>[2x]MHELTIYHFMSDKLNLYSDIGNIIALRQRAKKRNIKVNVVEINETEGITFDECDIFFIGGGSDREQALATKELSKIKTPLKEAIEDGMPGLTICGGYQFLGKKYITPDGTELEGLGILDFYTESKTNRLTGDIVIESDTFGTIVGFENHGGRTYHDFGTLGHVTFGYGNNDEDKKEGIHYKNLLGTYLHGPILPKNYEITDYLLEKACERKGIPFEPKEIDNEAEIQAKQVLIDRANRQKKSRLEHHHHHH;>MRQWTAIHLAKLARKASRAVGKRGTDLPGQIAR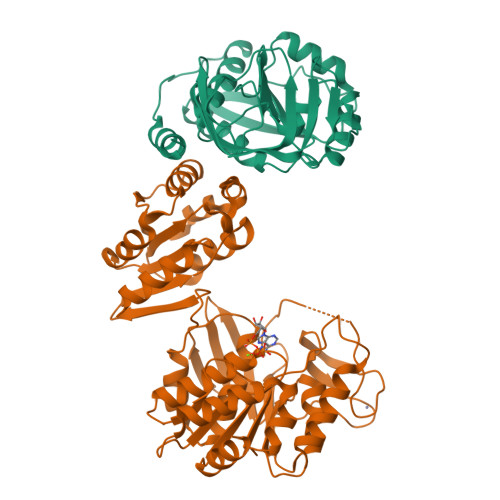KVDTDVLRKLAEQVDDIVFISGTNGKTTTSNLIGHTLKANNIQIIHNNEGANMAAGITSAFIMQSTPKTKIAVIEIDEGSIPRVLKEVTPSMMVFTNFFRDQMDRFGEIDIMVNNIAETISNKGIKLLLNADDPFVSRLKIASDTIVYYGMKAHAHEFEQSTMNESRYCPNCGRLLQYDYIHYNQIGHYHCQCGFKREQAKYEISSFDVAPFLYLNINDEKYDMKIAGDFNAYNALAAYTVLRELGLNEQTIKNGFETYTSDNGRMQYFKKERKEAMINLAKNPAGMNASLSVGEQLEGEKVYVISLNDNAADGRDTSWIYDADFEKLSKQQIEAIIVTGTRAEELQLRLKLAEVEVPIIVERDIYKATAKTMDYKGFTVAIPNYTSLAPMLEQLNRSFEGGQS[2x]>MNEKNIKHGQNFLIDTNILNRIVDHAEVTEKTGVIEIGPGIGALTEQLAKRAKKVVAFEIDQRLLPILKDTLSPYENVTVIHQDVLKADVKSVIEEQFQDCDEIMVVANLPYYVTTPIIMKLLEEHLPLKGIVV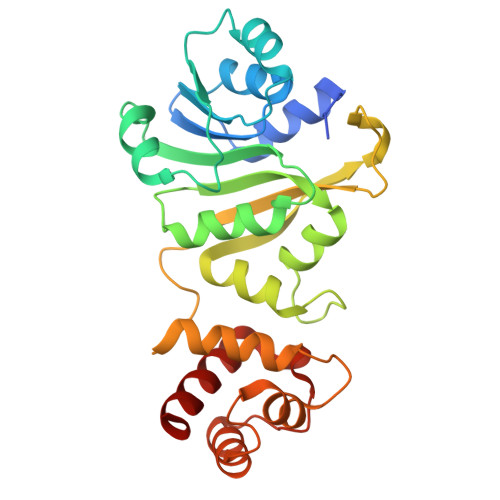MLQKEVAERMAADPSSKEYGSLSIAVQFYTEAKTVMIVPKTVFVPQPNVDSAVIRLILRDGPAVDVENESFFFQLIKASFAQRRKTLLNNLVNNLPEGKAQKSTIEQVLEETNIDGKRRGESLSIEEFAALSNGLYKALF[2x]> RVRSITLGNSTITTQECANVVVGYGVWPEYLKDNEATAEDQPTQPDVATCRFYTLESVQWMKNSAGWWWKLPDALSQMGLFGQNMQYHYLGRTGYTIHVQCNASKFHQGCLLVVCVPEAEMGCSNLNNTPEFAELSGGDTARMFTDTQIGETNSKKVQTAVWNAGMGVGVGNLT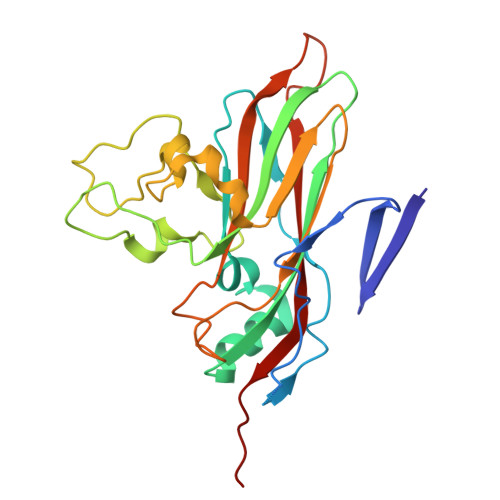IYPHQWINLRTNNSATIVMPYINSVPMDNMFRHNNLTLMIIPFVPLNYSEGSSPYVPITVTIAPMCAEYNGLRLA> HMKWTPPRSPFNLVQEILFHDPWKLLIATIFLNRTSGKMAIPVLWEFLEKYPSAEV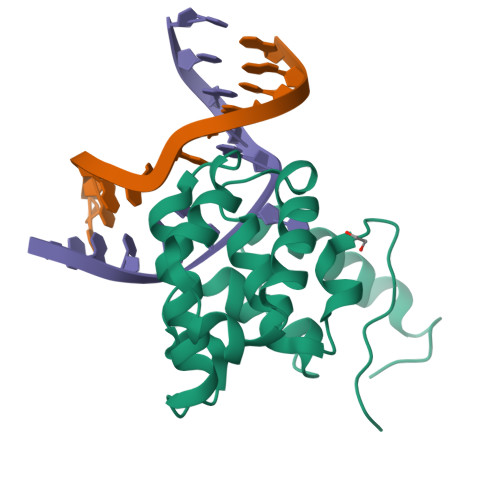ARAADWRDVSELLKPLGLYDLRAKTIIKFSDEYLTKQWRYPIELHGIGKYGNDSYRIFCVNEWKQVHPENHKLNKYHDWLWENHEKLSLS Native SAD (single-wavelength anomalous diffraction) is a de novo macromolecular structure-determination method in which the phase problem is solved by exploiting the anomalous diffraction signal of light atoms present in the crystal. Here, the combined use of these two strategies is described to solve cases of native SAD phasing that were particular challenges: the integral membrane diacylglycerol kinase (DgkA) with a low Bijvoet ratio of 1% and the large 200 kDa complex of the CRISPR-associated endonuclease (Cas9) bound to guide RNA and target DNA crystallized in the low-symmetry space group C2. Here, we present two challenging native SAD cases solved by collecting low-dose data at multiple orientations from three crystals each: the integral membrane diacylglycerol kinase DgkA (Li et al., 2013; 2 × 42 kDa asymmetric unit, space group P212121, 2.6 Å resolution) and the large Cas9–RNA–DNA complex (Anders et al., 2014; 200 kDa asymmetric unit, space group C2, 2.2 Å resolution). Here, we show that multi-crystal averaging of data sets used in conjunction with a low-dose, multi-orientation strategy is beneficial in difficult cases where data from one crystal are insufficient.

The integral membrane diacylglycerol kinase DgkA has two trimers in the asymmetric unit representing 6 × 130 residues with a total molecular weight of 84 kDa. Previous SAD and MAD attempts at the Zn absorption edge were unsuccessful. The structure was originally solved by Se-SAD phasing at the Se peak using crystals diffracting to 2.05 Å resolution. The crystals used in the current study only diffracted to 2.6 Å resolution (see §2.1.1). Data were collected both with and without multiple crystal orientations. Analysis of the substructure data exemplifies the weakness of the anomalous data, mainly owing to the disordered Met66 and Cys41 in chains E and F. The experimental Bijvoet ratio of 1% for this sample was therefore lower than the expected theoretical value of 1.1%.

>[6x]GHHHHHHELANNTTGFTRIIKAAGYSWKGLRAAWINEAAFRQEGVAVLLCVVIAAWLDVDAVTRVLLISSVMLVMIVELLNSAIEAVVDRIGSEYHELSGRAKDLGSAAVLIAIIDAVITWAILLWSHFG N-(pyridin-3-yl)pyrrolo[2,1-f][1,2,4]triazin-4-amine 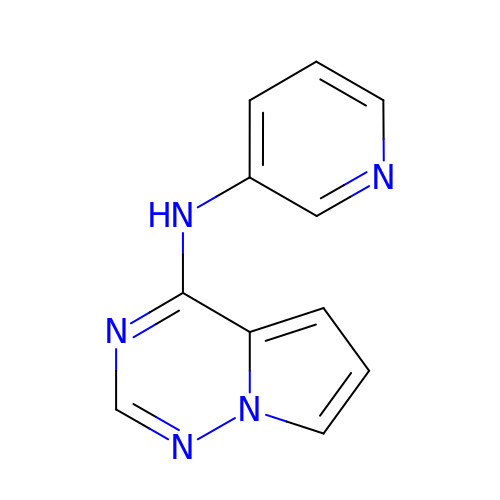| C11 H9 N5 | KTWGHBNFKBORPM-UHFFFAOYSA-N>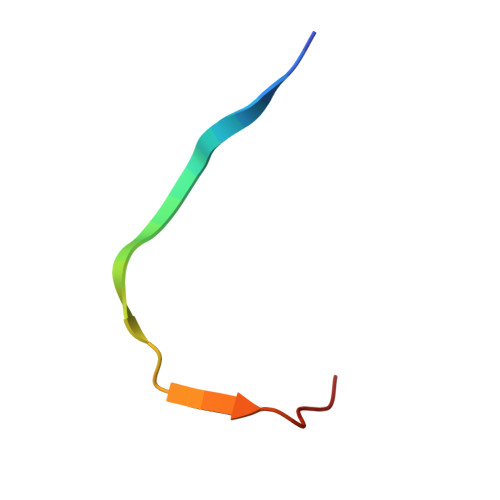 MTFEMLYSKIHRATITDANLNYIG>[2x]NDKLTLWTTPAPSPNCRLNAEKDAKLTLVLTKCGSQILATVSVLAVKGSLAPISGTVQSAHLIIRFDENGVLLNNSFLDPEYWNFRNG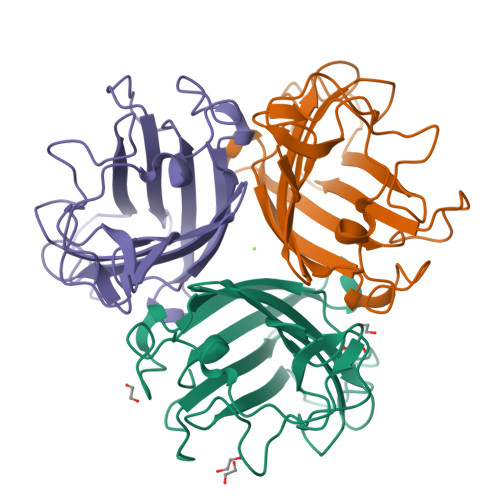DLTEGTAYTNAVGFMPNLSAYPKSHGKTAKSNIVSQVYLNGDKTKPVTLTITLNGTQETGDTTPSAYSMSFSWDWSGHNYINEIFATSSYTFSYIAQE;> KNNDKLTLWTTPAPSPNCRLNAEKDAKLTLVLTKCGSQILATVSVLAVKGSLAPISGTVQSAHLIIRFDENGVLLNNSFLDPEYWNFRNGDLTEGTAYTNAVGFMPNLSAYPKSHGKTAKSNIVSQVYLNGDKTKPVTLTITLNGTQETGDTTPSAYSMSFSWDWSGHNYINEIFATSSYTFSYIAQE Proliferating cell nuclear antigen (PCNA) is a fundamental protein involved in maintaining genome integrity, with roles in both DNA replication and repair. PCNA is a trimeric, ring-shaped molecule with pseudo-hexagonal symmetry that can accommodate double-stranded DNA through a central pore. PCNA and other processivity factors tether polymerases to DNA to increase their processivity and are commonly referred to as sliding clamps. Each processivity factor monomer possesses one binding pocket for a PIP-box bearing protein.

To investigate the halophilic adaptation of such a key protein we have crystallised and solved the structure of Haloferax volcanii PCNA (HvPCNA) to a resolution of 2.0 Å. The crystal structure of HvPCNA was solved to 2.0 Å resolution and contains one trimer in the asymmetric unit. The overall architecture is very similar to other known PCNA structures, as expected. 274 water molecules and nine sodium ions are modelled in the asymmetric unit. Analysis using the PISA server shows that the buried surface area at the HvPCNA interface is relatively small at 1160 Å2 (averaged over the ncs related subunits). HvPCNA also has a relatively small interface and so forms just five main chain hydrogen bonds, with further side chain interactions involving Asp172 OD2 with Tyr106 OH and Ala109 N. The net charge, calculated assuming histidines to be neutral, of HvPCNA is -31, considerably higher than the remaining PCNA structures (-13 to -20). HvPCNA is markedly different from typical sliding clamps, with almost total loss of the usual positive surface charge in the inner pore. Examination of the inner ring reveals that HvPCNA possesses only two basic residues (per monomer), Lys143 and Lys205, that extend into the channel and are likely to contribute significantly to the postulated water-mediated interactions with the phosphate backbone of DNA passing through the pore. The principle cation binding site is located around a carboxylate cluster (Asp146, Asp150 and Asp198), towards the inner edge of the ring and appears to contain two Na+ ions coordinated by the carboxylate groups, water molecules and main chain carbonyls.

>[3x]MFKAIVSAATLRDALDSVSVLVDECKIRLNEESLSIRAVDPANVGMVDLTLDAAAFESYEAHGGVIGVNLSRLEEVAGMAGAGDLIHLTLDEETRKLNIRIDGLSYTLALIDPDSIRQEPDIPDLDLAANIVLEGTHLDRGIKAADMVSDHIRLRVDGAEETFHIEAEGDTDDVDLSLPPADLISIEAGAADSLFSLDYLKDMNKAIPTDAEVTVELGEEFPVKLHYQIAEGMGTITYMLAPRIQSD>MNLIPTVIEQTSRGERAYDIYSRLLKDRIIMLGSAIDDNVANSIVSQLLFLDAQDPEKDIFLYINSPGGSISAGMAIYDTMNFVKADVQTIGMGMAASMGSFLLTAGANGKRFA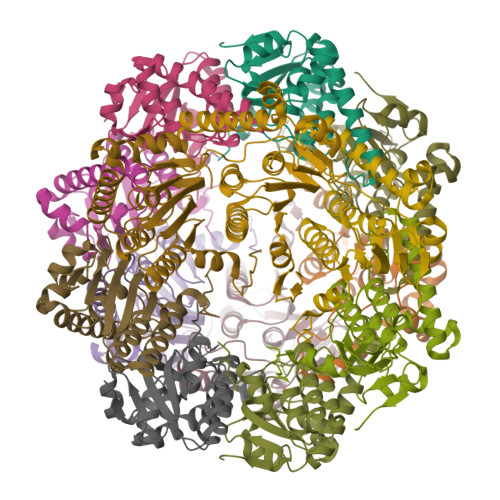LPNAEIMIHQPLGGAQGQATEIEIAARHILKIKERMNTIMAEKTGQPYEVIARDTDRDNFMTAQEAKDYGLIDDIIINKSGLKGMASWSHPQFEK[7x]> MTNKVVILGSTNVDQFLTVERYAQPGETLHVEEAQKAFGGGKGANQAIATARMQADTTFITKIGTDGVADFILEDFKVAHIDTSYIIKTAEAKTGQAFITVNAEGQNTIYVYGGANMTMTPEDVINAKDAIINADFVVAQLEVPIPAIISAFEIAKAHGVTTVLNPAPAKALPNELLSLIDIIVPNETEAELLSGIKVTNEQSMKDNANYFLSIGIKTVLITLGKQGTYFATKNQSQHIEAYKVNAID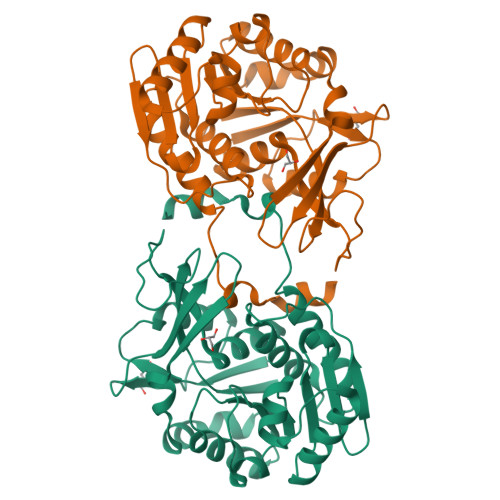TTAAGDTFIGAFVSRLNKSQDNLADAIDFGNKASSLTVQKHGAQASIPLLEEVNQV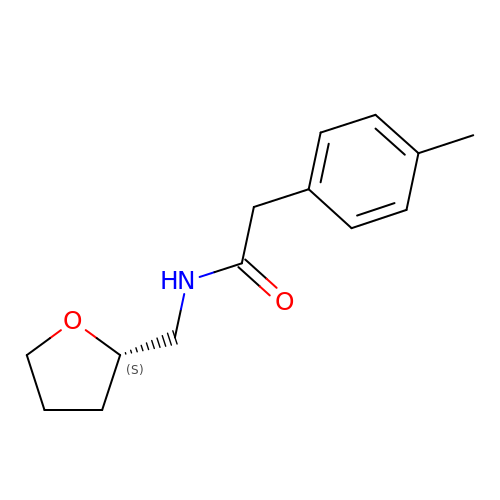2-(4-methylphenyl)-N-{[(2S)-oxolan-2-yl]methyl}acetamide | C14 H19 N O2 | GNNODMPIMQHVQL-ZDUSSCGKSA-N>GHMDELFEEHLEIAKALFAQRLPYWCDVFLRPADQAFNAYLNARGQASTYLVLEGFDPVYVPRGCDLDAVRATARARA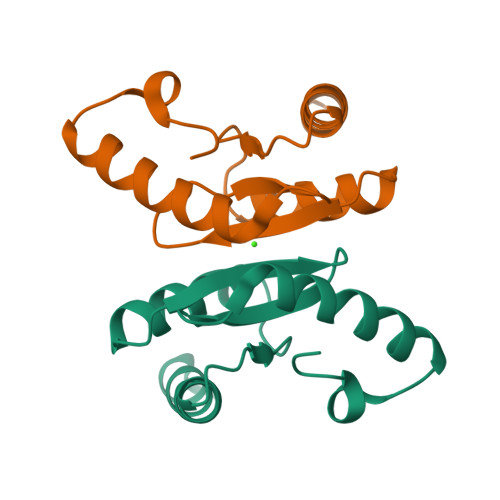RLREAGLGEDALPVLL[2x]>MIIYRDLISHDELFSDIYKIREIADGLCLEVEGKMVSRTEGAIDDSLIGGNASAEGPEGEGTESTVVTGVDIVMNHHLQETSFTKEAYKKYIKDYM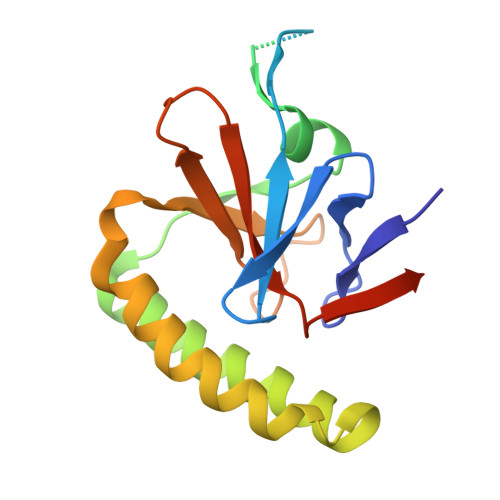KSLKGKLEEQKPERVKPFMTGAAEQIKHILANFNNYQFFIGENMNPDGMVALLDYREDGVTPFMIFFKDGLEMEKCLEHHHHHH[2x]> PGSVVELLGKSYPQDDHSNLTRKVLTRVGRNLHNQQHHALWL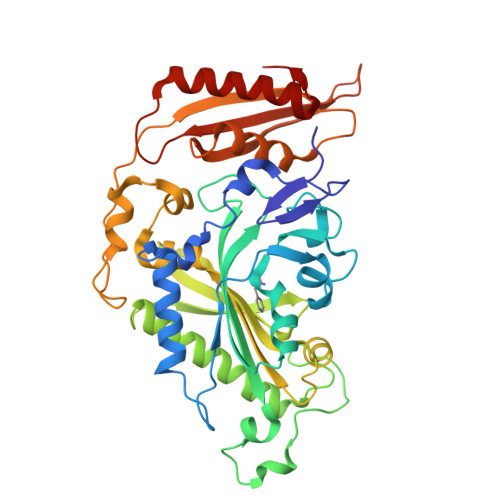IKERVKEHFYKQYVGRFGTPLFSVYDNLSPVVTTWQNFDSLLIPADHPSRKKGDNYYLNRTHMLRAHTSAHQWDLLHAGLDAFLVVGDVYRRDQIDSQHYPIFHQLEAVRLFSKHELFAGIKDGESLQLFEQSSRSAHKQETHTMEAVKLVEFDLKQTLTRLMAHLFGDELEIRWVDCYFPFTHPSFEMEINFHGEWLEVLGCGVMEQQLVNSAGAQDRIGWAFGLGLERLAMILYDIPDIRLFWCEDERFLKQFCVSNINQKVKFQPLSKYPAVINDISFWLPSENYAENDFYDLVRTIGGDLVEKVDLIDKFVHPKTHKTSHCYRITYRHMERTLSQREVRHIHQALQEAAVQLLGVEGRF> AEPVIDTDGNPLHRGGKYYIMPSIWGPPGGGLRLGKTENLNCPVTVLQDYSEVINGLPVEFNIRGILPRTIFTDTELNIEFTEKPNCAENSRWSLFEDDKIHKAYVGIGDS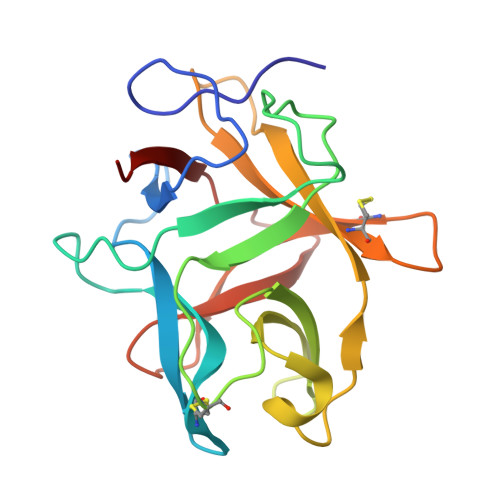EDHPDQEMLSGSFYIKKHGLRNNTYKLVFCRDGSSTCSDIGRYDNNEDGRRLILTADLPYEVVFVNAS>SLSRTVHHQQTAEITQQAADFIRYMNAINDY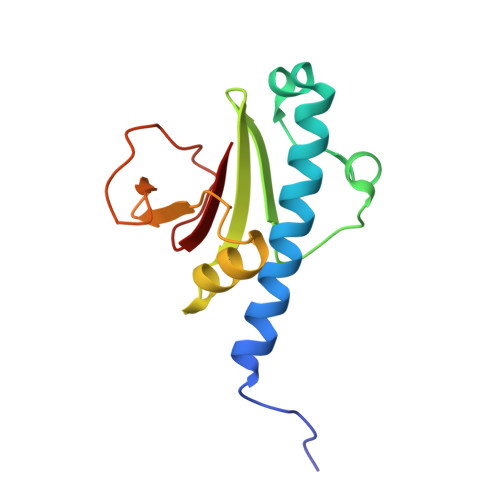LYQHPERRAAGGQLTSAQLGLPATKNVSHLISQQRVFVWAKEKPGLMGALLEQSGDSALLARVENGRLLDTHGRRISITLPAVIPDQVIIWMN[2x]> GSPESFPDAHMRMILRKPPGQRTVDDLEIIYDELLHIKALSHLSTTVKRELAGVLIFESHAKGGTVLFNQGEEGTSWYI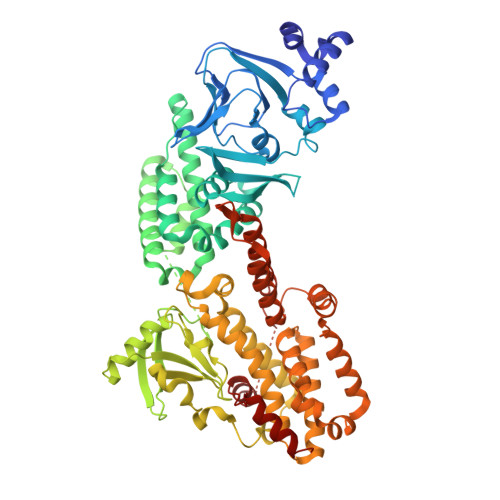ILKGSVNVVIYGKGVVCTLHEGDDFGKLALVNDAPRAASIVLREDNCHFLRVDKEDFNRILRDVEANTVRLKEHDQDVLVLEKVPAGNRAANQGNSQPQQKYTVMSGTPEKILEHFLETIRLEPSLNEATDSVLNDFVMMHCVFMPNTQLCPALVAHYHAQPSQGTEQERMDYALNNKRRVIRLVLQWAAMYGDLLQEDDVAMAFLEEFYVSVSDDARMMAAFKEQLPELEKIVKQISEDAKAPQKKHKVLLQQFNTGDERAQKRQPIRGSDEVLFKVYCIDHTYTTIRVPVAASVKEVISAVADKLGSGEGLIIVKMNSGGEKVVLKSNDVSVFTTLTINGRLFACPREQFDSLTPLPEQEGPTTGTVGTFELMSSKDLAYQMTTYDWELFNCVHELELIYHTFGRHNFKKTTANLDLFLRRFNEIQFWVVTEVCLCSQLSKRVQLLKKFIKIAAHCKEYKNLNSFFAIVMGLSNVAVSRLALTWEKLPSKFKKFYAEFESLMDPSRNHRAYRLTAAKLEPPLIPFMPLLIKDMTFTHEGNKTFIDNLVNFEKMRMIANTARTVRYYRSQPFNPDAAQANKNHQDVRSYVRQLNVIDNQRTLSQMSHRLEPRRP> PITVIVSGATGFIAQHVVKQLLAKNYQVIGTVRSTAK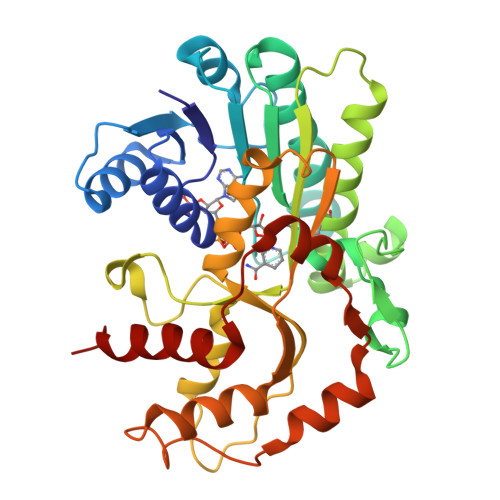GDHLLKLFNNPKNLSYEIVEDVGTKGAFDKVLQKHGEAKVFLHLASPFHFNVTDVEKELLLPAVDGTKNVLQAIYNFGNNIEKVVITSSYAAISTASKEADKNAIITEKDWNEISWQDALLNPVNGYRGSKKFAEKAAWDFIKSNDNVKFSLSTINPSFVFGPQSFGSEIKQSLNTSSEIINSILKLKPNDSIPASKGGWVDVRDVAKAHIIAFENEDAKNQRILLNSGRFTSQSLVDIINDKFPDLKGKIPVDPGSDKSVIAESLATIDDTKSRELLGFEYYNLEQSVYDTVEQIVNAHK>MTAASIDRELVPWSDPEFRNNPYPWYRRLQQDHPVHKLEDGTYLVSRYADVSHFAKLPIMSVEPGWADAGPWAVASDTALGSDPPHHTVLRRQTNKWFTPKLVDGWVRTTRELVGDLLDGVEAGQVIEARRDLAVVPTHVTMARVLQLPEDDADAVMEAMFEAMLMQSAEPADGDVDRAAVAFGYLSARVAEMLEDKRVNPGDGLADSLLDAARAGEITESEAIATILVFYAVGHMAIGYLIASGIELFARRPEVFTAFRNDESARAAIINEMVRMDPPQLSFLRFPTEDVEIGGVLIEAGSPIRFMIGAANRDPEVFDDPDVFDHTRPPAASRNLSFGLGPHSCAGQIISRAEATTVFAVLAER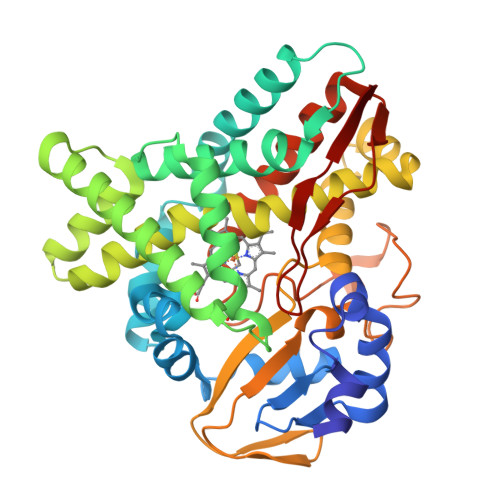YERIELAEEPTVAHNDFARRYRKLPIVLS[2x]> GPLGSMEGEELIYHNIINEILVGYIKYYINDISEHELSPYQQQIKKILTYYDECLNKQVTITFSLTSVQEIKTQFTGVVTELFKDLINWGRICGFIVF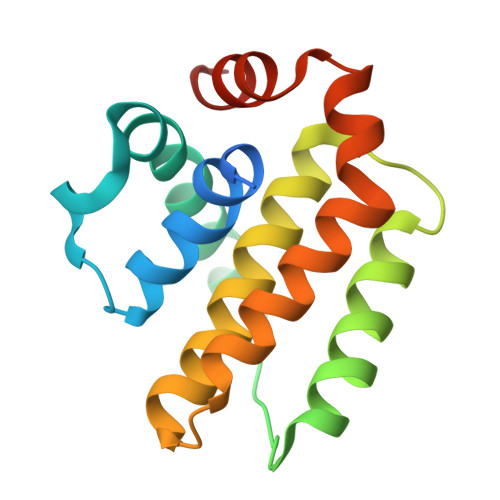SAKMAKYCKDANNHLESTVITTAYNFMKHNLLPWMISHGGQEEFLAFSLHSDMYS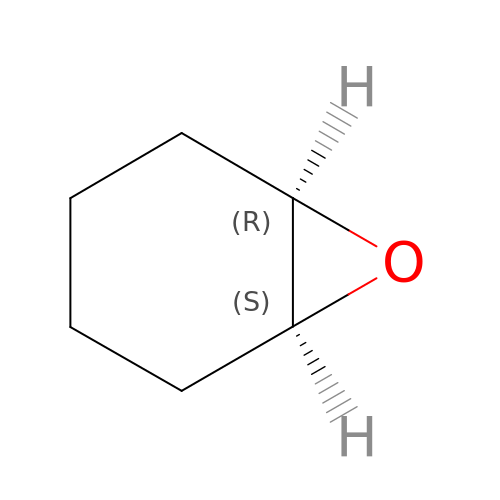(1R,6S)-7-oxabicyclo[4.1.0]heptane | C6 H10 O | ZWAJLVLEBYIOTI-OLQVQODUSA-N>[2x]EAVVISGRKLAQQIKQEVRQEVEEWVASGNKRPHLSVILVGENPASHSYVLNKTRAAAVVGINSETIMKPASISEEELLNLIN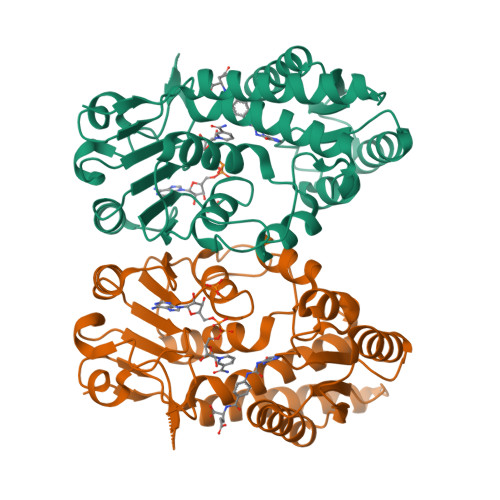KLNNDDNVDGLLVQLPLPEHIDERRICNAVSPDKDVDGFHVINVGRMCLDQYSMLPATPWGVWEIIKRTGIPTLGKNVVVAGRSKNVGMPIAMLLHTDGAHERPGGDATVTISHRYTPKEQLKKHTILADIVISAAGIPNLITADMIKEGAAVIDVGINRVHDPVTAKPKLVGDVDFEGVRQKAGYITPVPGGVGPMTVAMLMKNTIIAAKKVLRLEEREVLKSKELGVATN(2S)-1-oxo-1-[(4-sulfamoylphenyl)amino]propan-2-yl (2S)-2-methyl-1,2,3,4-tetrahydroacridine-9-carboxylate 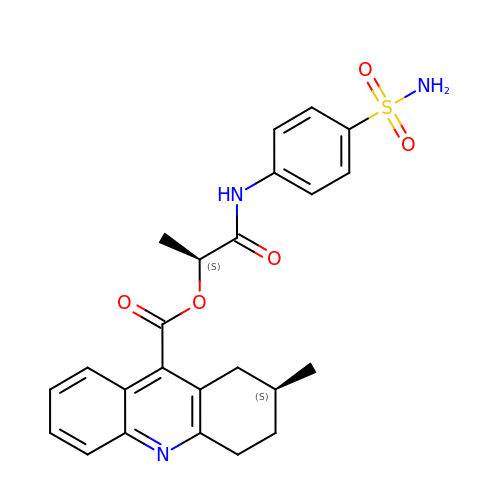| C24 H25 N3 O5 S | ZICDFSXBQFNQBM-GJZGRUSLSA-N> MPKHEFSVDMTCGGCAEAVS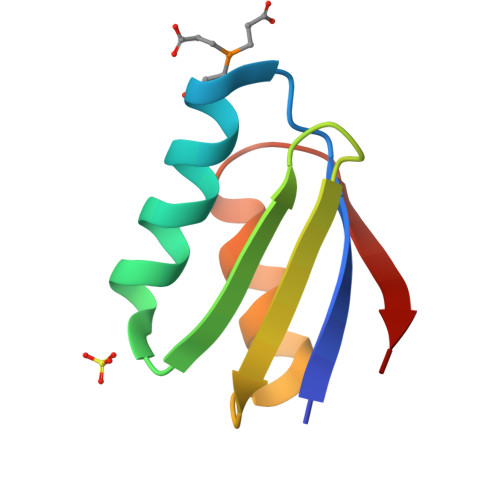RVLNKLGGVKYDIDLPNKKVCIESEHSMDTLLATLKKTGKTVSYLGLE(((S)-1-carboxy-5-((E)-2-cyano-3-(5-(1-(3-methoxy-3-oxopropyl)-1,2,3,4-tetrahydroquinolin-6-yl)thiophen-2-yl)acrylamido)pentyl)carbamoyl)-L-glutamic 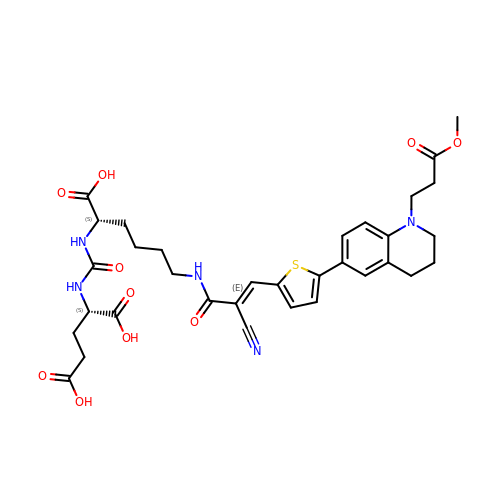acid | C33 H39 N5 O10 S | UBYIMALNFXGAEL-ITFMGPALSA-N>[4x]DPVEDGLVIETDSGPVEIVTKTAPPAFLADTFDTIYSGWHFRDDSTRDLERDDFD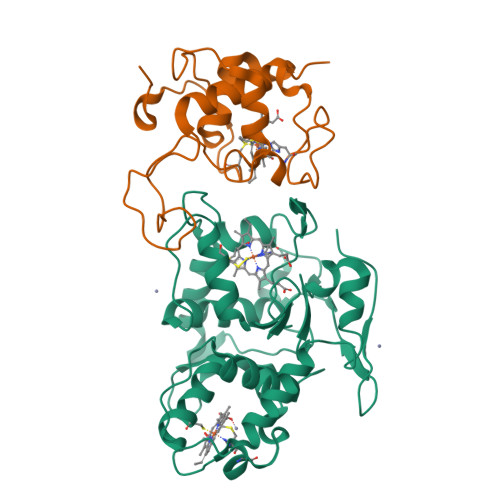NPAMVFVDRGLDKWNAAMGVNGESCASCHQGPESMAGLRAVMPRVDEHTGKLMIMEDYVNACVTERMGLEKWGVTSDNMKDMLSLISLQSRGMAVNVKIDGPAAPYWEHGKEIYYTRYGQLEMSCANCHEDNAGNMIRADHLSQGQINGFPTYRLKDSGMVTAQHRFVGCVRDTRAETFKAGSDDFKALELYVASRGNGLSVEGVSVRH;>[4x]CETAPKEVVYVEGAVEASLTGAPGNPEEGVRIMTTNALGNCVACHQIGALPDVEFPGTIAPPLDGAGDRWTEAQLRGIVANAKMTFEGTFMPAFYKVDGFVRPGDGFSGKAGAEPLAPILNAQQIEDVVAFLVTLKE>MAMITGGELVVRTLIKAGVEHLFGLHGSHIDTIFQACLDHDVPIIDTRHEAAAGHAAEGYARAGAKLGVALVTAGGGFTNAVTPIANAWLDRTPVLFLTGSGALRDDETNTL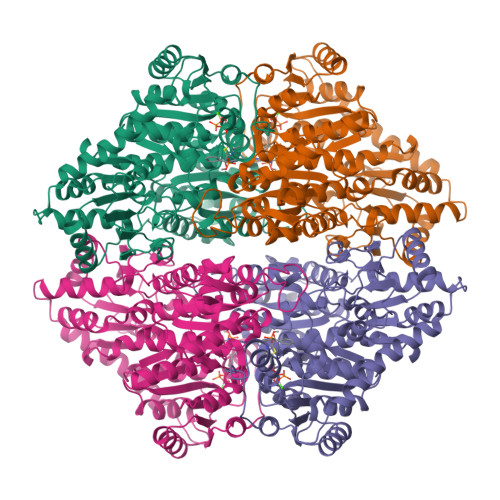QAGIDQVAMAAPITKWAHRVMATEHIPRLVMQAIRAALSAPRGPVLLDLPWDILMNQIDEDSVIIPDLVLSAHGARPDPADLDQALALLRKAERPVIVLGSEASRTARKTALSAFVAATGVPVFADYEGLSMLSGLPDAMRGGLVQNLYSFAKADAAPDLVLMLGARFGLNTGHGSGQLIPHSAQVIQVDPDACELGRLQGIALGIVADVGGTIEALAQATAQDAAWPDRGDWCAKVTDLAQERYASIAAKSSSEHALHPFHASQVIAKHVDAGVTVVADGALTYLWLSEVMSRVKPGGFLCHGYLGSMGVGFGTALGAQVADLEAGRRTILVTGDGSVGYSIGEFDTLVRKQLPLIVIIMNNQSWGATLHFQQLAVGPNRVTGTRLENGSYHGVAAAFGADGYHVDSVESFSAALAQALAHNRPACINVAVALDPIPPEELILIGMDPFGSHHHHHH[2x]> MLDNLAVHPEQLPPRPWITLKERDQILPSASFTVMCYNVLCDKYATRQLYGYCPSWALNWEYRKKGIMEEIVNCDADIISLQEVETEQYFTLFLPALKERGYDGFFSPKSRAKIMSEQERKHVDGCAIFFKTEKFTLVQKHTVEFNQVAMANSDGSEAMLNRVMTKDNIGVAVVLEVHKELFGAGMKPIHAADKQLLIVANAHMHWDPEYSDVKLIQTMMFVSEVKNILEKASSRPGSPTADPNSIPLVLCADLNSLPDSGVVEYLSNGGVADNHKDFKELRYNEC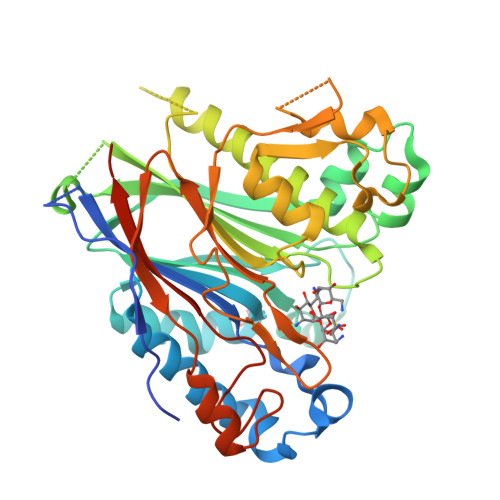LMNFSCNGKNGSSEGRITHGFQLKSAYENNLMPYTNYTFDFKGVIDYIFYSKTHMNVLGVLGPLDPQWLVENNITGCPHPHIPSDHFSLLTQLELHPPLLPLVNGVHLPNRR>[4x]MDSYQLFLDGEFVDAADGRTFTTTDPGNEQPVATVAQAGEADALRAIEAARWAFDHGEWPKMTPQERAARIYDFADHVTKLAGRLAMAESMDAGHVINLSKFWAANGAALLRNLAHYSANSFPWEEEIPYSGNVGAPGRDYIRREPIGVCVGIIPWNFPASMAFWKISHAIIMGNTIVLKPATQTPLTALIIAEAAKAAGIPKGVINVITGQGREVGNLLCTHPDVDKISFTGSTSVGNNIMKLAADSTKRVTLELGGKSANIILDDADLDAAVEGAVFGTFLHQGQVCESGTRLLVSSKIYDAFIDKLKARTEALRVGYPLSPESHLGPLVSGKQLETVE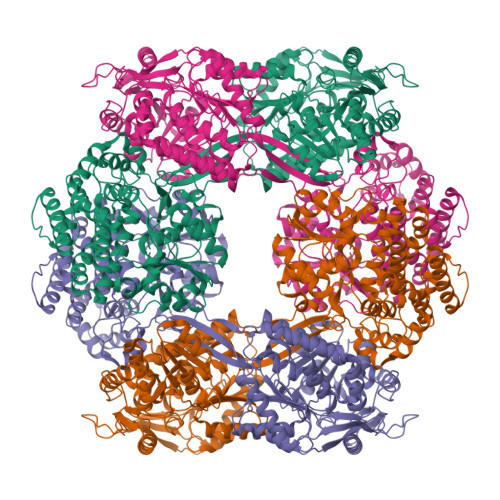GYVKLGLEEGATLLTGGHRVEVPGISGGHYYAPTIFTDVDNRMRIAQEEIFGPVVVVIRFDSDEEAVAIANDSIYGLAGGVYSGSNARAQRVATQLRTGTVWINNYHAFGDFCPFGGYKQSGFGREMGASGLSEFVQVKRVHVSAYASVGASPAMAILSDDKKTPFVQYNAPTNIISGHGSLPAIYKEMVKLGCKRAVIMTDEGVNATGLPTLVREALDDFCVGVYDRIEQDSSLDTVDAAAAYARECGADAIVSVGGGSVIDTSKAVCVVLKNGGKCNDHMAMLRLQEPQTPHIAIPTTSGTGSEVTNVAVIKNKAVGRKVYILDPHIVPNSTILDPRFTLGLPHRMTVTTALDAMTHSIEALTSTRSQPICDGQALQAIRLISENLPRVVAKPHDEAARANLQLAATMAGWAFNVAQVGLAHAMAHTLGAIHDIPHGLACGIMLPRVMRFNVDHAGHKLALAAQALGVQTTGMDAREAGLAAAQAVEALMQSVDHPRYLSDLGVPRDNLSNLAAHAMGDAAIMFNARPVKGPQEVMAVYEEAY>MSLADAVAHLTPERWEEANRLLVRKALAEFTHERLLTPEREPDDGGGQTYVVRSDDGQTAYRFTATVRALDHWQVDAASVTRHRDGAELPLAALDFFIELKQTLGLSDEILPVYLEEISSTLSGTCYKLTKPQLSSAELARSGDFQAVETGMTEGHPCFVANNGRLGFGIHEYLSYAPETASPVRLVWLAAHRSRAAFTAGVGIEYESFVRDELGAATVDRFHGVLRGRGLDPADYLLIPVHPWQWWNKLTVTFAAEVARGHLVCLGEGDDEYLAQQSIRTFFNASHPGKHYVKTALSVLNMGFMRGLSAAYMEATPAINDWLARLIEGDPVLKETGLSIIRERAAVGYRHLEYEQATDRYSPYRKMLAALWRESPVPSIREGETLATMASLVHQDHEGASFAGALIERSGLTPTEWLRHYLRAYYVPLLHSFYAYDLVYMPHGENVILVLADGVVRRAVYKDIAEEIAVMDPDAVLPPEVSRIAVDVPDDKKLLSIFTDVFDCFFRFLAANLAEEGIVTEDAFWRTVAEVTREYQESVPELADKFERYDMFAPEFAL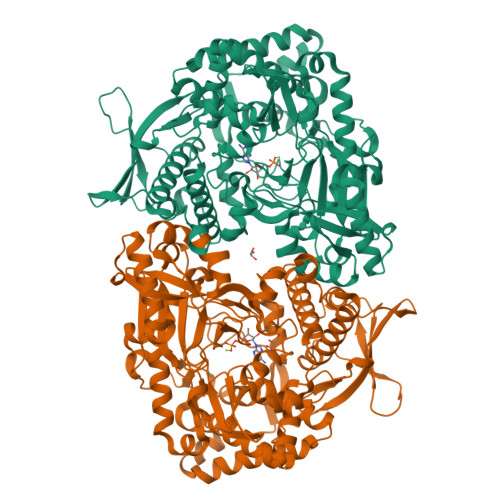SCLNRLQLRDNRQMVDLADPSGALQLVGTLKNPLAGR[4x]3-[(1S)-1,2,3,4-Tetrahydronapthalen-1-ylamino)-2,5,6-trifluoro-4-[(2-hydroxyethyl)sulfonyl]benzenesulfonamide 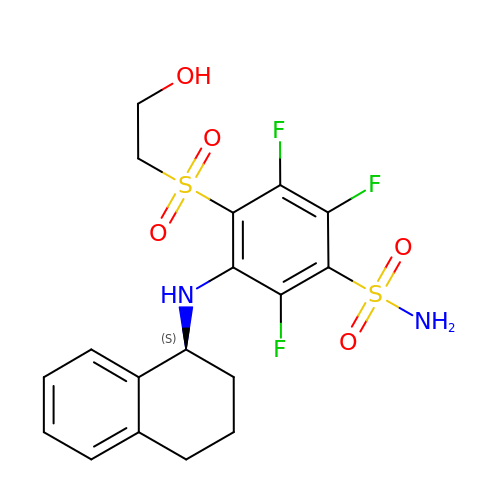| C18 H19 F3 N2 O5 S2 | FFYQSPGIPXYOLF-LBPRGKRZSA-N4-(2,6-dimethoxyphenoxy)-2,6-dimethoxyphenol 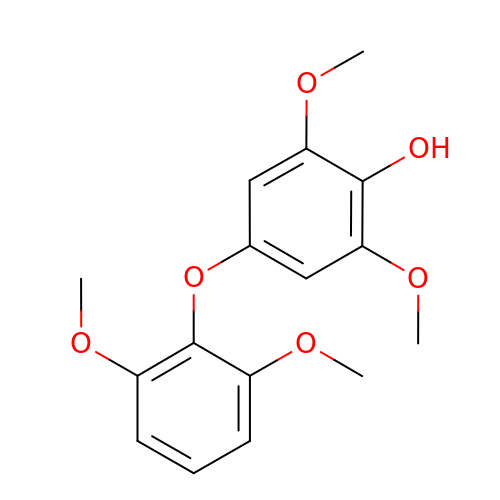| C16 H18 O6 | JKALBPJYUOVWCR-UHFFFAOYSA-N>MAHHHHHHMGNNEKGAIFRSLHRAGQPLALFNVWDAGSARVVADAGAVALATGSWSVAAANGFVDGEQMPRALMMEVLERIVRATDLPVTVDLESGYGERPEDVAETIAMSIRAGAIGCNLEDSFPSTGELRDVDEAAARIAAARQAADRAGVDYFINARTDVFFKAATETHDERLLDATLARARAYAAAGADGLFVPGLRSPALIRALTAASPLPVNVMRVAET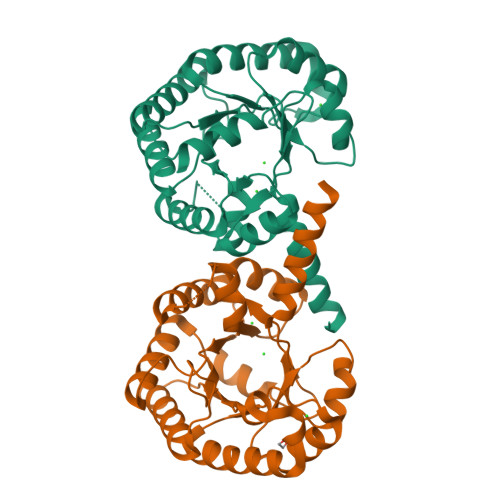PTLAELAEYGVARISHGPYPYLQAMKTLAALVKQGG[8x]>SGGGDGSTYSAEIRRTTMGVPHIKAGNWGSAGYGFGYVQAQDNLCTMADSFLTYRGERSRHLGGSAQLVYNSTLGRPRNIDSDFFHRHVISDEAVDRTMAAQPAKLLQMVEGFAAGYNRYVREAKAGGSAHAACRSEAWVQPITARDVWRRIYAANLAGGYSNFAEAIANAQPPQAKAGAQEPAAFEPGRTRAPSLQGSNMYGFGTAATGEGSGVLFGNPHWYWKGPDRFYQAQLTIDGEANVSGVSFLGLPVIQIGFNDSVAWSHTVSTARRFGFFQLSLVQGEPTSYLRDGVPVKMKPATITVPSRNADGSVSDVTRTLYHSEFGPLVNLAGLNPALAWSQGTAFAIRDINGENFRTLRTWMRWNQAKSLDEFIAIQKEEASIPWVNTVAVGRGSAKAWYADIGAVPNVSPAQTAACTTPFGMAVGQALPNVPFFDGSRSECDWLTDADSVQKGAVGVSRMPSLQRDDYVGNMNDSYWLANVHAPLTGYPAIFGPAGTSAQTLRTRMGHTMALERLAGTDGYAGNKATSAVVREMVLGSRVFSAERFKDEVLDLICTPAQWTVNGAAVDAAQACAVLAAWDNRGRKDSRGSHLWDEFWSRVPTASLFTVPFSAADPLNTPRGINAAAADALRQAMATAIARVGQSGYALDAPRGEVLYATRGGTRLPLYGGCGAMGYFTITCSENDITQGGYSMDGQPNASNSYMQVVSFPASGVQAHTFLTFSLSDDPASPHHGDYTKAYSAGQWLRVPFTEAEITGNADYRTATVKELEHHHHHH[4x]

The recombinant MacQ protein exhibited bifunctional acylase activity against various ranges of AHLs and against multiple β-lactam antibiotics, including penicillin G, ampicillin, and amoxicillin. The MacQ protein is comprised of 806 amino acid residues, including an N-terminal signal peptide, and belongs to the N-terminal nucleophile (Ntn) hydrolase superfamily. AHL-acylase is one of the enzymes capable of inactivating AHLs via hydrolysis of the amide bond of the acyl side-chain to produce homoserine lactone (HSL) and fatty acid. The MacQ structure clearly revealed a typical Ntn-hydrolase fold comprised of a four-layered α-β-β-α motif45 mainly composed of two polypeptide chains, α- and β-chains, generated by self-cleaving activity.

On the basis of the previous reports regarding CA, we created an SP-shortened MacQ by deleting seven residues from Val20SP to Val26SP (from Val203 to Val209). Unexpectedly, SDS-PAGE analysis showed that the purified SPΔ7 was uncleaved and was present as a single polypeptide chain with a subunit weight of approximately 80 kDa, suggesting that the seven-residue deletion of the SP inactivated the self-cleaving maturation, despite the fact that SPΔ7 possesses the catalytic serine (Ser1β in the cleaved form). Interestingly, SPΔ7 exhibited unambiguous degrading activity against almost all of the substrates tested for wild-type MacQ. We successfully determined the crystal structure of MacQ SPΔ7 in ligand-free form. However, each molecule was determined to be a homodimer composed of two uncleaved SPΔ7 polypeptides. The overall structure of SPΔ7 superimposed very well on that of the wild-type enzyme without its SP region. We could build the continuous atomic model for chain A, while several residues corresponding to the SP region of the wild-type enzyme were disordered for the chain B, and most of the residues of the SP region (residue 179–200) were disordered for chains C and D. The conformation of the SP region of the SPΔ7 (residue 183–202) was found to be completely different from that of the SP in the wild-type enzyme. The structure of SPΔ7 indicates a possible mechanism of the autoproteolytic cleavage between Gly202 and Ser203. In the SPΔ7 structure, the ~3.4 Å distance between the main-chain O of Gly202 and the main-chain amide of Val272 would be too distant to form a hydrogen bond. However, the pocket is insulated from the solvent because of the presence of the uncleaved polypeptide chain (residues Leu201-Ser203).>MEFSSFLFTILLFSLNISPLVSAHGSNHEDFLKCLSYRMNDNTVEPKVIHTSKDSSFFSILDSSIQNPRFSVSETPKPVSIITPVKASDVQTVIRCAQLHGIHVRTRSAGHCYEGLSYIAYNKPFAVIDLRNLRSISLDVDNRTGWVQTGATAGELYYEIGKTTKSLAFPAGIHPTVGVGGQFSGGGYGTLLRKYGLAADNIIDALVVDASGRILDRQAMGEDYFWAIRGGGGSSFGVILSWKVKLVDVPSTITVFKVQKTSKKEAVRIIKKWQYAADKVPDDLFIRTTLERSNKNAVHALFTGLYIGPVNNLLALMEEKFPELGLEKEGCEEMSWIESVLWFADFPKGESLGVLTNRERTSLSFKGKDDFVQEPIPEAAIQEIWRRLEAPEARLGKIILTPFGGKMSEMAEYETPFPHRGGNLYEIQYVAYWREEEDKNKTETDKYLKWVDSVYEFMTPYVSKSPRGAYVNFKDMDLGMYLGKKKTKYEEGKSWGVKYFKNNFERLVRVKTRVDPTDFFCDEQSIPLVNKVT[2x]

Among these, the flavin-dependent oxidoreductases berberine bridge enzyme-like enzymes stand out, because of the bi-covalent attachment of the cofactor to the protein via a histidine and a cysteine. Here we report the crystallographic structure of AtBBE-like 28, a member of the type II BBE-like enzyme sub-family. AtBBE-like 28 functions in biomass formation and salt stress tolerance.

Crystallization was conducted using the sitting-drop method, yielding crystals diffracting to a resolution of 1.8 Å. In the case of AtBBE-like 28, the cysteine is replaced by His174, which does not form a covalent bond to the C6-position. However, the covalent linkage established by the conserved GGHD motif was clearly seen in the crystal structure (His111 in Fig 3). The flavin adopts a butterfly-bent shape, with an angle at the N5-N10 axis of 6°. Asp369 and Glu426 are found at a distance of 2.4 Å, indicating that they share a proton. An additional interesting feature of the active site is the proton-relay established between the putative catalytic base, Tyr188, and the neighboring acidic side chains of Glu426 and Asp369, which presumably activate Tyr188 to facilitate proton abstraction. In AtBBE-like 28, this position is occupied by Val177 and thus we assume that the pocket is available for oxygen binding. In agreement with this assumption, an electron density in this pocket was clearly detectable and we propose that a chloride ion, acting as an oxygen surrogate, is bound to the pocket (green sphere). The distance between the chloride and the C(4a) of the isoalloxazine ring is 3.1 Å. AtBBE-like 28 features a hydrogen bond donor to N(5) (Nπ of His174) and a catalytic base to initiate substrate oxidation (Tyr188) and hence shares the hallmarks of a flavoprotein oxidase, as proposed by Fraaije and coworkers.Zinc is essential for virulence and survival and is acquired solely by the ABC transporter, AdcCB, and two Zn2+-specific cluster A-I SBPs, AdcA and AdcAII, in S. pneumoniae. Although both SBPs share this structural core, AdcA also has a C-terminal domain (residues 322 to 501; here termed AdcAC) that is structurally related to ZinT, a periplasmic protein from E. coli and Salmonella. The AdcAC domain is linked to the N-terminal cluster A-I domain of AdcA (residues 1 to 311, henceforth referred to as AdcAN) by an 11-amino-acid linking region. Collectively, our data show that the AdcAN domain is necessary and sufficient for Zn2+ acquisition, with the AdcAC domain and the His-rich loop aiding in Zn2+ recruitment during growth under Zn2+-restricted conditions.

The AdcAN domain has a two-lobed organization, with the N- and C-terminal (α/β)4 lobes bisected by a cleft in which the metal binds. The binding site in AdcAN is comprised of three Nε2 atoms from His63, His140, and His204 and one Oε2 atom from Glu279. These four residues bind a single Zn2+ ion via 4-coordinate geometry, with bond distances of 1.98 to 2.08 Å. Intriguingly, the AdcAN domain was observed in a conformation that partially exposed the metal-binding site to bulk solvent, with the relative solvent accessibility of the metal-binding residues (His63 > His140 > His204 ≈ Glu279) remaining the same during the five independent MD simulations. The partial opening of the Zn2+-binding site of the AdcAN domain arises from the α7β6 loop having moved away from the binding site due to rigid-body rotational movements of α7 in a plane perpendicular to the helical hinge interlobe helix α5. This conformation was also observed for the truncated AdcA variant that lacked AdcAC, AdcAN (residues 27 to 309). The high-resolution crystal structure of Zn2+-bound truncated AdcAN did not reveal any conformational differences by comparison with the N-terminal domain of the full-length, wild-type protein. Metal binding was restricted to Zn2+ ions, with differential scanning fluorimetry (DSF) showing that other divalent first-row transition metal ions did not induce stabilization of the N-terminal domain. In the AdcAN domain, the metal-binding site is located beneath the surface of the protein and is largely preformed in the absence of ligand. This permits the bioinorganic chemistry of the site to be tightly defined and likely aids in achieving selectivity for Zn2+ over other metal ions.

>GKLNIVTTFYPVYEFTKQVAGDTANVELLIGAGTEPHEYEPSAKAVAKIQDADTFVYENENMETWVPKLLDTLDKKKVKTIKATGDMLLLPGGEEEEGDHDHGEEGHHHEFDPHVWLSPVRAIKLVEHIRDSLSADYPDKKETFEKNAAAYIEKLQSLDKAYAEGLSQAKQKSFVTQHAAFNYLALDYGLKQVAISGLSPDAEPSAARLAELTEYVKKNKIAYIYFEENASQALANTLSKEAGVKTDVLNPLESLTEEDTKAGENYISVMEKNLKALKQTTDQEGPAIEPEKAEDTKTV[4x]> MTTRLEWAKASPDAYAAMLGLEKALAKAGLERPLIELVYLRTSQINGCAYCVNMHANDARKAGETEQ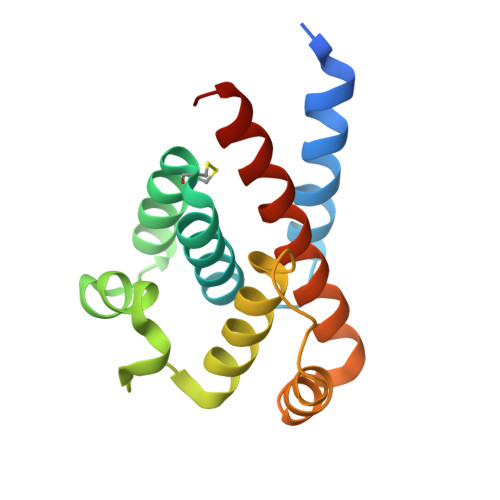RLQALCVWQETPYFTPRERAALAWTEQLARLSQGPLPHGLLDELREHFDDKEIAELTLAVSAINAWNRFGVGMGMQPE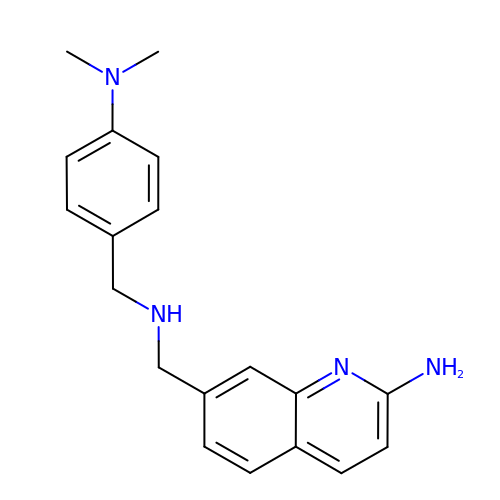7-[({[4-(dimethylamino)phenyl]methyl}amino)methyl]quinolin-2-amine | C19 H22 N4 | JEOSSXMVBYPUED-UHFFFAOYSA-N(1R,2R)-N-(1-cyanocyclopropyl)-2-[(8-fluoro-1,3,4,5-tetrahydro-2H-pyrido[4,3-b]indol-2-yl)carbonyl]cyclohexanecarboxamide 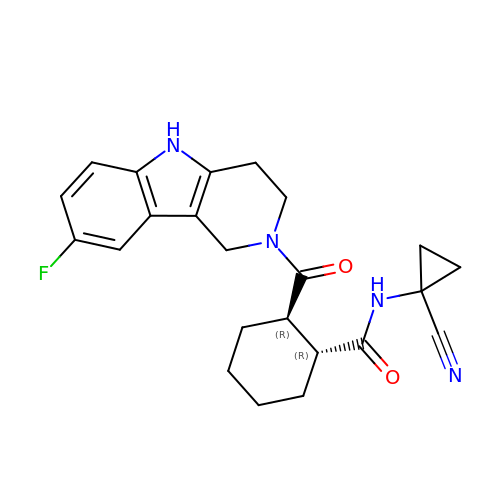| C23 H25 F N4 O2 | HGJTURTZFKNELD-HZPDHXFCSA-N>[12x]FARSLSITTPEEMIEKAKGETAYLPCKFTLSPEDQGPLDIEWLISPADNQKVDQVIILYSGDKIYDDYYPDLKGRVHFTSNDLKSGDASINVTNLQLSDIGTYQCKVKKAPGVANKKIHLVVLV;>[12x]MRGSHHHHHHGSPPAAPITLWTGPGPSINGFINDTPVIRCFICLTRDSNLVTVNASFVGEGGYRIVSPTQSQFSLIMEFDQFGQLMSTGNINSTTTWGEKPWGNNTVQP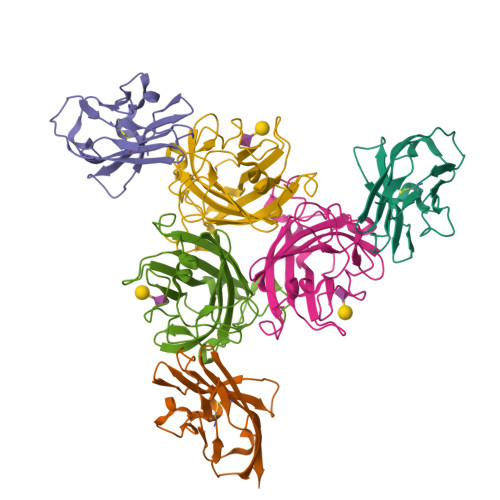RPSHTWKLCMPNREVYSTPAATISRCGLDSIAVDGAPSRSIDCMLIINKPKGVATYTLTFRFLNFNRLSGGTLFKTDVLTFTYVGENQ>GSEFQNKNFRAPQSEAIGILYKLIETGSKHKNMYDHTEITTDSLLALLGSEKVKIIDVRSADAYNGWRMRGEVRGGHIKGAKSLPAKWLTDPEWLNIVRFKQIRPEDAIVLYGYTPEECEQTATRFKENGYNNVSVFHRFHPDWTGNDAFPMDRLEQYNRLVPAEWVNGLISGEEIPEYDNDTFIVCHAHYRNRDAYLSGHIPGATDMDTLALESPETWNRRTPEELKKALEEHGITASTTVVLYGKFMHPDNADEFPGSAAGHIGAIRLAFIMMYAGVEDVRVLNGGYQSWTDAGFAISKDDVPKTTVPEFGAPIPSRPEFAVDIDEAKEMLQSEDSDLVCVRSYPEYIGEVSGANYIKKKGRIPGAIFAECGSDAYHMENYRNHDHTTREYHEIEDIWAKSGIIPKKHLAFYCG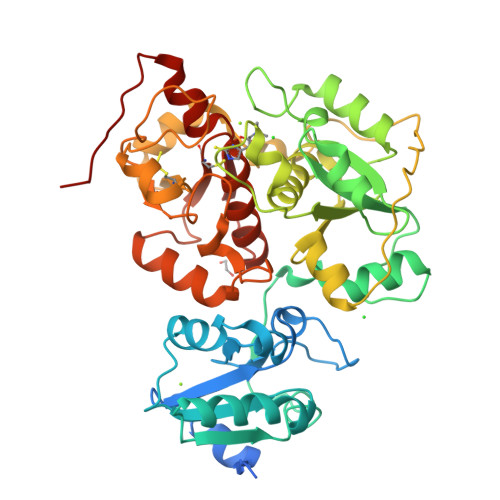TGWRGSEAWFNALLMGWPRVSVYDGGWFEWSNDPENPYETGVPK[2x]>[2x]GKDGSNSLAEIRTDFNILYSMMKKHEEF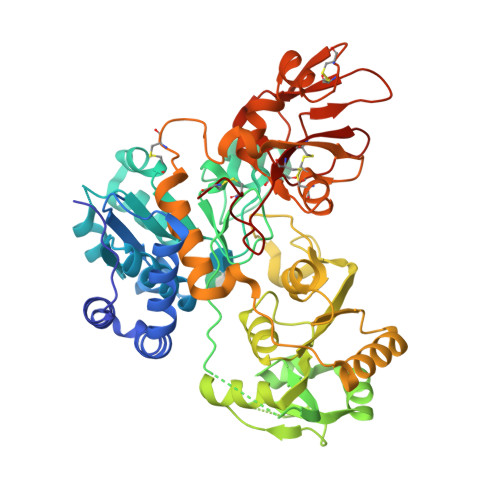RWMRLRIRRMADAWIQAIKSLAEKQNLEKRKRKKVLVHLGLLTKESGFKIAETAFSGGPLGELVQWSDLITSLYLLGHDIRISASLAELKEIMKGGGGIVELIYIDIVGLAQFKKTLGPSWVHYQCMLRVLDSFGTEPEFNHANYAQSKGHKTPWGKWNLNPQQFYTMFPHTPDNSFLGFVVEQHLNSSDIHHINEIKRQNQSLVYGKVDSFWKNKKIYLDIIHTYMEVHATVYGSSTKNIPSYVKNHGILSGRDLQFLLRETKLFVGLGFPYEGPAPLEAIANGCAFLNPKFNPPKSSKNTDFFIGKPTLRELTSQHPYAEVFIGRPHVWTVDLNNQEEVEDAVKAILNQKIEPYMPYEFTCEGMLQRINAFIEKQDFCHGQVMWPPLSALQVKLAEPGQSCKQVCQESQLICEPSFFQHLNKDKDMLKYKVTCQSSELAKDILVPSFDPKNKHCVFQGDLLLFSCAGAHPRHQRVCPCRDFIKGQVALCKDCL>MADKRIRSDSSAA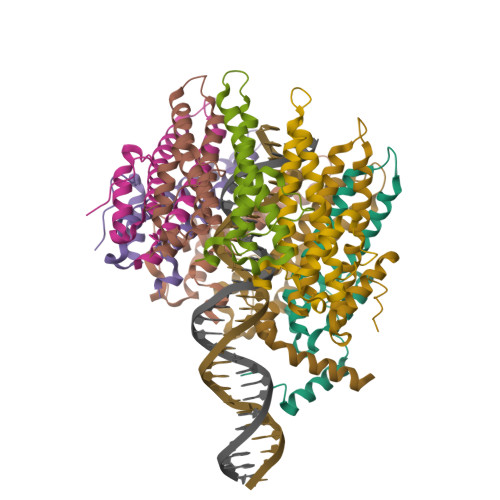AVQAMKNAAVDTIDPPSHAGLEKKAEPFWHDNIRSKALDSWTPADLLAAVELANNQLYITVLRKDLRKEERIRGEERDEGLIKDLRKQIVELQRTILAQRRDLQIHSHATNGESRDQKKRNQNDRDARNTKNEHQDQDDNLIAFPKHG[9x]> ASMTGGQQMGRGSSLTACPEESPLLVGPMLIEFNIPVDLKLVEQQNPKVKLGG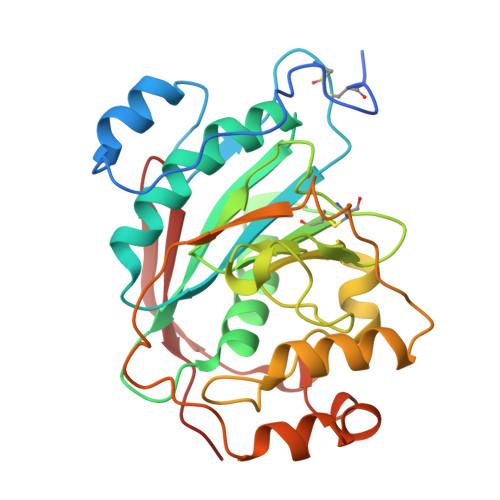RYTPMDCISPHKVAIIIPFRNRQEHLKYWLYYLHPILQRQQLDYGIYVINQAGESMFNRAKLLNVGFKEALKDYDYNCFVFSDVDLIPMNDHNTYRCFSQPRHISVAMDKFGFSLPYVQYFGGVSALSKQQFLSINGFPNNYWGAGGEDDDIYNRLAFRGMSVSRPNAVIGKTRMIRHSRDKKNEPNPQRFDRIAHTKETMLSDGLNSLTYMVLEVQRYPLYTKITVDIGTPS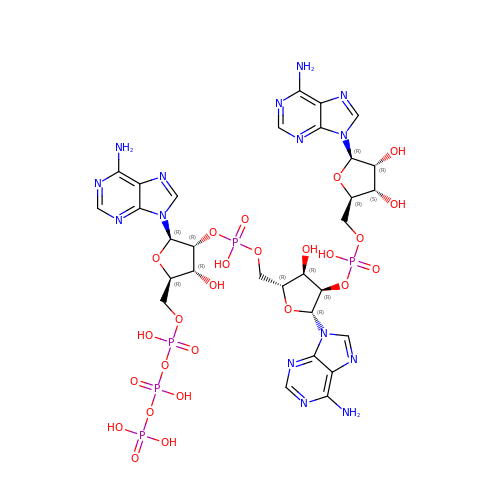[[(2R,3R,4R,5R)-5-(6-aminopurin-9-yl)-4-[[(2R,3R,4R,5R)-5-(6-aminopurin-9-yl)-4-[[(2R,3S,4R,5R)-5-(6-aminopurin-9-yl)-3,4-dihydroxy-oxolan-2-yl]methoxy-hydroxy-phosphoryl]oxy-3-hydroxy-oxolan-2-yl]methoxy-hydroxy-phosphoryl]oxy-3-hydroxy-oxolan-2-yl]methoxy-hydroxy-phosphoryl] phosphono hydrogen phosphate | C30 H40 N15 O25 P5 | RTAGLZBJCCVJET-UQTMIEBXSA-N>VIEKVQHIQLLQKNVRAQLVDMKRLEVDIDIKIRSCRGSCSRALAREVDLKDYEDQQKQLEQVIAK[2x];>[2x]HQLYIDETVNSNIPTNLRVLRSILENLRSKIQKLESDVSAQMEYCRTPCTVSCNIPVVSGKECEEIIRKGGETSEMYLIQPDSSVKPYRVYCDMNTENGGWTVIQNRQDGSVDFGRKWDPYKQGFGNVATNTDGKNYCGLPGEYWLGNDKISQLTRMGPTELLIEMEDWKGDKVKAHYGGFTVQNEANKYQISVNKYRGTAGNALMDGASQLMGENRTMTIHNGMFFSTYDRDNDGWLTSDPRKQCSKEDGGGWWYNRCHAANPNGRYYWGGQYTWDMAKHGTDDGVVWMNWKGSWYSMRKMSMKIRPFFPQQ;>[2x]YEASILTHDSSIRYLQEIYNSNNQKIVNLKEKVAQLEAQCQEPCKDTVQIHDITGKDCQDIANKGAKQSGLYFIKPLKANQQFLVYCEIDGSGNGWTVFQKRLDGSVDFKKNWIQYKEGFGHLSPTGTTEFWLGNEKIHLISTQSAIPYALRVELEDWNGRTSTADYAMFKVGPEADKYRLTYAYFAGGDAGDAFDGFDFGDDPSDKFFTSHNGMQFSTWDNDNDKFEGNCAEQDGSGWWMNKCHAGHLNGVYYQGGTYSKASTPNGYDNGIIWATWKTRW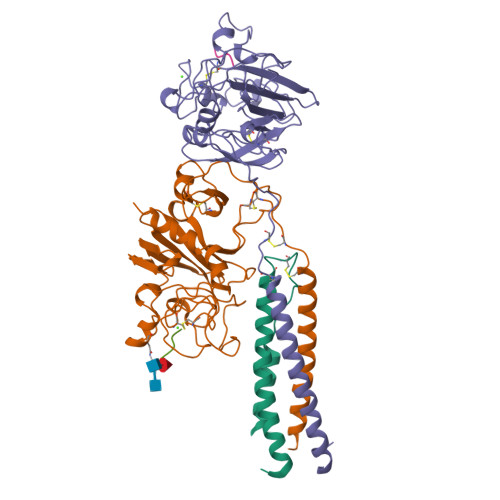YSMKKTTMKIIPFNRLTIGEGQQHHLGGAK;>GPRP[2x];>[2x]GHRP>GEFKGLMAVGLAEHDKEAWGRLPFSLTIADISQDDEPLIYVNRAFEQMTGYSRSSVVGRNCRFLQGEKTDPGAVERLAKAIRNCEEVEETIYNYRADGEGFWNHLLMGPLEDQDEKCRYFVGIQVDMGQSESPDRATELD[4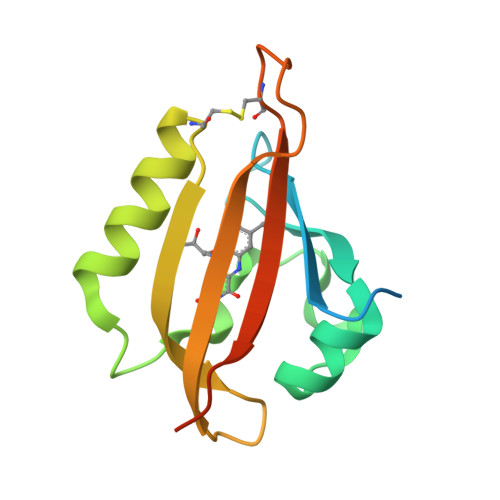x]> TPDCVTGKVEYTKYNDDDTFTVKVGDKELF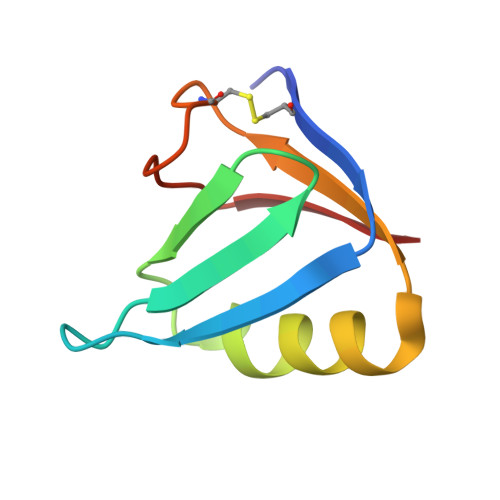TNRWNLQSLLLSAQITGMTVTIKTNACHNGGGFSEVIFR> AQVI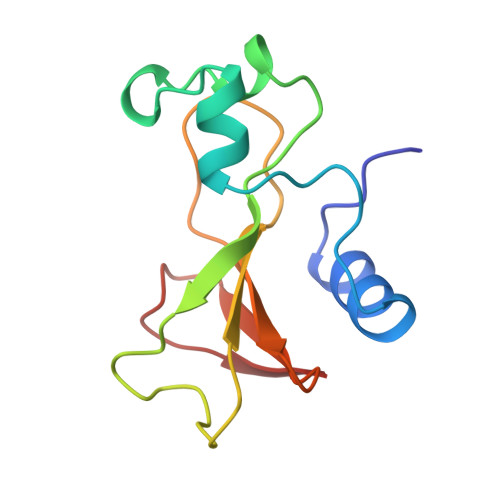NTFDGVADYLQTYHKLPDNYITASEAQALGWVASKGNLADVAPGKSIGGDIFSNREGKLPGKSGRTWREADINYTSGFRNSDRILYSSDWLIYKTTDHYQTFTKIR>[4x]MIPDDEFIKNPSVPGPTAMEVRCLIMCLAEPGKNDVAVDVGCGTGGVTLEL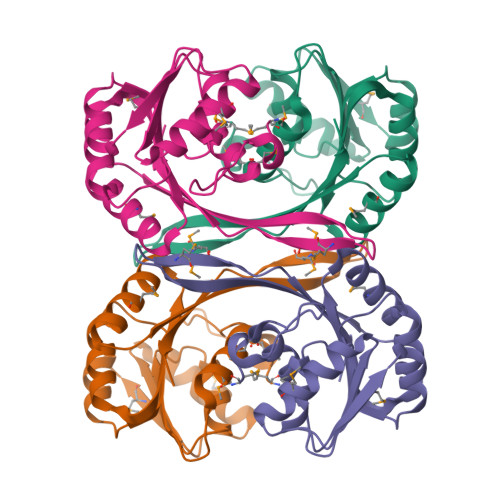AGRVRRVYAIDRNPEAISTTEMNLQRHGLGDNVTLMEGDAPEALCKIPDIDIAVVGGSGGELQEILRIIKDKLKPGGRIIVTAILLETKFEAMECLRDLGFDVNITELNIARGRALDRGTMMVSRNPVALIYTGVSHENKD However, a dormant state in Firmicutes can be recapitulated in the laboratory. This paper describes the first structure of a group of peptidoglycan cleaving enzymes from Firmicutes, called stationary phase survival proteins (Sps), that are involved in survival in the stationary phase and are analogous to the resuscitation promoting factors (Rpfs) from Actinobacteria. In this paper we present three high-resolution crystal structures of YuiC, an Sps protein from B. subtilis. The overall fold of each domain of the symmetric dimer consists of a mixed direction six stranded double psi beta barrel surround by five helices. In all the structures, the final two helices and the last strand of the beta barrel of each half are supplied by the other chain in the dimer.

The apo structure forms a similar dimer to that seen in the R3 structure (in this case with the dimeric symmetry axis corresponding to the crystallographic two fold axis parallel to the unit cell b axis). In the apo crystals, the two fold axis is crystallographic. The apo structure is locally less ordered than the substrate bound structures, lacking density for residues 97–100 and for four residues at the C-terminus compared to the + NAG structure, which just misses one residue at the C-terminus. Otherwise, the apo form of the pseudo monomer superposes well onto the + NAG structure with an RMSD of 1.15 Å over 135 CA atoms for the pseudo monomer. The domain swapped dimers superimpose less well with the RMSD for the apo dimer vs + NAG of 2.81 Å over 241 CA atoms as a consequence of flexibility in the positioning of the pseudo monomers within the dimer. The NZ of K178 in the apo structure forms hydrogen bonds to both the main chain and side chain carbonyls of N173, whereas in the liganded structures this side chain is pointing in to solvent. The region 176–178 lies away from the sugar binding site, so the change is not a direct result of ligand binding. However the other end of the third helix lies quite close to the ligand binding site and the loop that becomes ordered on ligand binding, so the difference in domain position may be propagated from sugar binding.

> PLEEAFDWDEYPVQRVTATGYTAGAESTGKNPGDPLYGLTYSGVKVKRDLYSTVAADPSVFPIGTILFIPNYGLGVVADTGSAIKGNRLDLYFETVKDVYNEWGKKTLDVYVIKKGTGKITEDELEKLNETKSLQVFRNQYKTVKE>[2x]GSGNVDLVFLFDGSMSLQPDEFQKILDFMKDVMKKLSNTSYQFAAVQFSTSYKTEFDFSDYVKRKDPDALLKHVKHMLLLTNTFGAINYVAT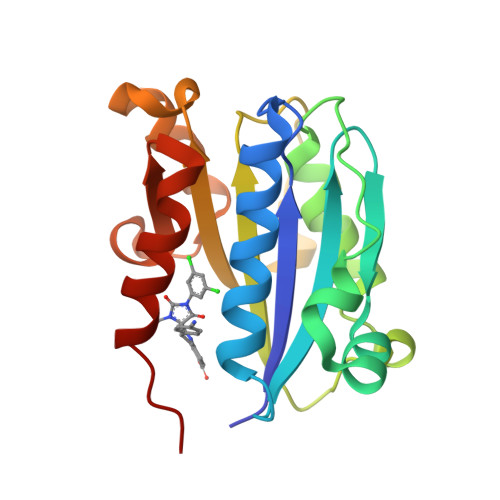EVFREELGARPDATKVLIIITDGEATDSGNIDAAKDIIRYIIGIGKHFQTKESQETLHKFASKPASEFVKILDTFEKLKDLFTELQKKIYVI>SHMNKKDLRSPICCILGHVDTGKTKLLDKIRQTNVQGGEAGGITQQIGATYFPIDAIKAKTKVMAEYEKQTFDVPGLLVIDTPGHESFSNLRSRGSSLCNIAILVIDIMHGLEQQTIESIKLLRDRKAPFVVALNKIDRLYDWKAIPNNSFRDSFAKQSRAVQEEFQSRYSKIQLELAEQGLNSELYFQNKNMSKYVSIVPTSAVTGEGVPDLLWLLLELTQKRMSKQLMYLSHVEATILEVKVVEGFGTTIDVILSNGYLREGDRIVLCGMNGPIVTNIRALLTPQPLRELRLKSEYVHHKEVKAALGVKIAANDLEKAVSGSRLLVVGPEDDEDELMDDVMDDLTGLLDSVDTTGKGVVVQASTLGSLEALLDFLKDMKIPVMS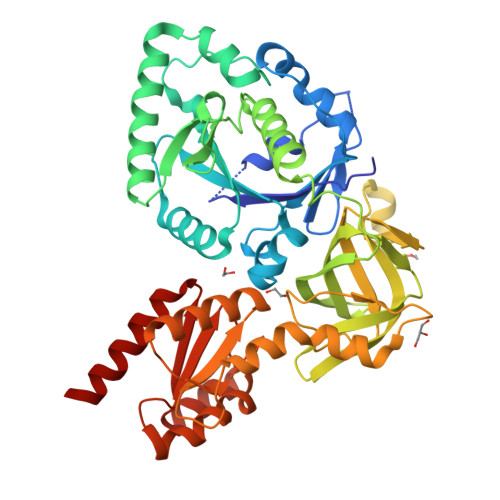IGLGPVYKRDVMKASTMLEKAPEYAVMLCFDVKVDKEAEQYAEQEGIKIFNADVIYHLFDSFTAYQEKLLE[2x]> MVSLPRMVYPQSKVLTPCRKDVLVVTPWLAPIVWEGTFNIDILNEQFRLQNTTIGLTVFAIKKYV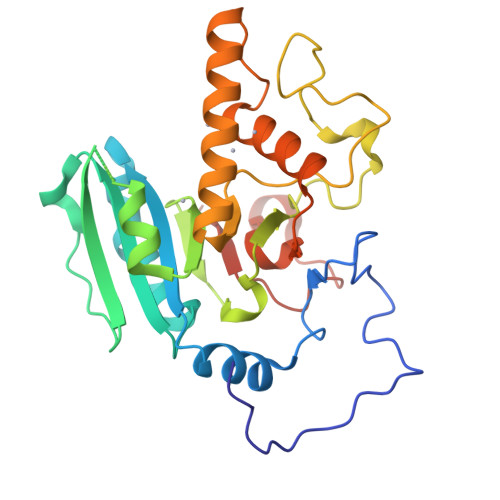AFLKLFLETAEKHFMVGHRVHYYVFTDQPAAVPRVTLGTGRQLSVLEVRAYKRWQDVSMRRMEMISDFCERRFLSEVDYLVCVDVDMEFRDHVGVEILTPLFGTLHPGFYGSSREAFTYERRPQSQAYIPKDEGDFYYLGGFFGGSVQEVQRLTRACHQAMMVDQANGIEAVWHDESHLNKYLLRHKPTKVLSPEYLWDQQLLGWPAVLRKLRFTAVPKNHQAVRNP>[6x]SNAERKEGEVAGLDMNISQFLKSLGLEHLRDIFETEQI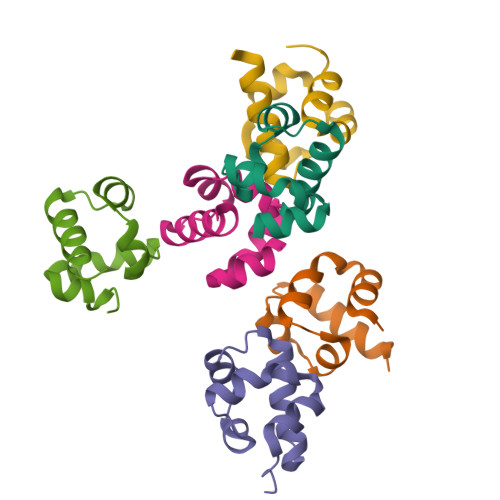TLRVLADMGHEELKEIGINAYGHRHKLIKGVERLLGGQQGT(3R,5R)-3-methoxy-5-(4-methoxyphenyl)-5-(3-pyridin-3-ylphenyl)-3,4-dihydropyrrol-2-amine 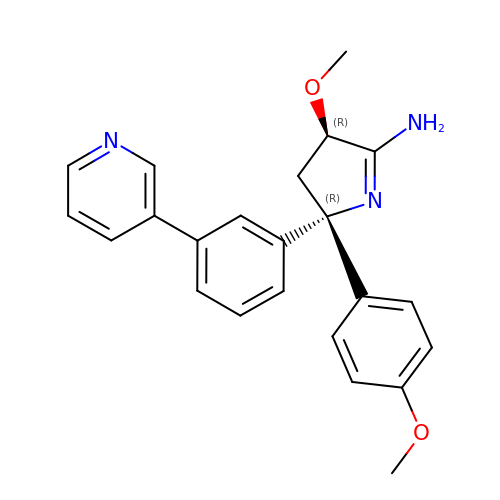| C23 H23 N3 O2 | XBWQSEBJKSPBBV-FYYLOGMGSA-N>[2x]NLEMEIILTLSQGLKKYYGKILKLLHLTLEEDTEGLLEWCKRNLGSNCDDDFFQKRIEEFFITGEGYFNEVLQFKTLSTPSSTEPSHARLPTAEPFKSYFAKGFLSIDSGYFSAKCYPRSSTSGLQLINVTQHPARIAETPGPKTTSLKTINCINLRASVFKEHREVEINVLLPQIAVNLSNCHVVINSHVCDYSLDTDGPVRLPRIYHEGTFMPGTYKIVIDRKNKLNDRCTLVTNCVIKGREVRKGQSVLRQYKTEIKIGKAPTGSLEVLFQ

Crimean-Congo Hemorrhagic Fever Virus (CCHFV), a tick-borne virus from the Nairoviridae family, causes hemorrhagic fever and death in 5–40% of cases. The GPC includes two structural glycoproteins (GN and GC) and secreted glycoprotein 38 (GP38) containing proteins that also can be linked to a mucin-like domain (MLD) and one non-structural protein (Nsm). The role of GP38 in viral replication and pathogenesis is still being elucidated, but GP38 is essential in the maturation of CCHFV particles. Additional studies have observed that GP38 may be secreted or localized to the outside of infected cells and the viral envelope.

One X-ray structure of GP38 from IbAr10200 has been solved, which has given initial insight into its overall fold, but a GP38-antibody complex has yet to be described. As only one structure of GP38 had been previously solved and was from clade III CCHFV IbAr10200, a highly laboratory-passaged strain with little clinical relevance, we solved an additional structure of GP38 from Clade V CCHFV Hoti. This human isolate is one of the two that can be used to elicit human disease-like symptoms in a non-human primate model. In addition, CCHFV Hoti has a 15% sequence identity difference with that of the IbAr10200 isolate that might reveal any major differences in tertiary structures or surface composition between CCHFV GP38s. Crystals of the CCHFV Hoti GP38 were readily obtained, and the structure was solved to a resolution of 3.2 Å. Both the structures of GP38 originating from the IbAr10200 and Hoti strains followed the same global fold. However, an additional alpha helix is detected between Hoti GP38 beta strands 2 and 3 near the N-glycosylation sites. Also, a divergent loop conformation is observed in amino acid region 490–500, and like the IbAr10200 structure no electron density for the amino acid region 330–345.1-[5-[2-[(4-azanylpiperidin-1-yl)methyl]-1,3-thiazol-4-yl]-4-ethyl-2-methyl-1~{H}-pyrrol-3-yl]ethanone | C18 H26 N4 O 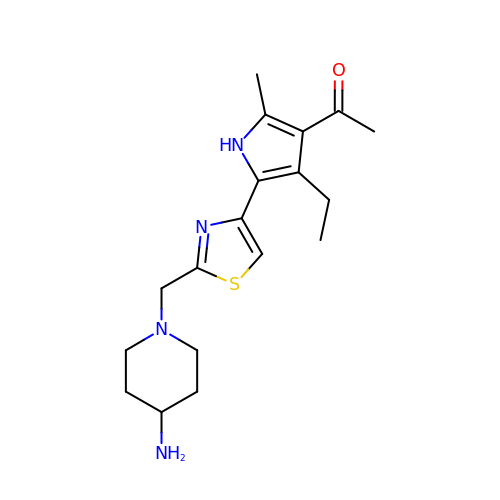S | XYCAHFXOGWMTBZ-UHFFFAOYSA-N>KSCPSVCRCDAGFIYCNDRSLTSIPVGIPEDATTLYLQNNQINNVGIPSDLKNLLKVQRIYLYHNSLDEFPTNLPKYVKELHLQENNIRTITYDSLSKIPYLEELHLDDNSVSAVSIEEGAFRDSNYLRLLFLSRNHLSTIPGGLPRTIEELRLDDNRISTISSPSLHGLTSLKRLVLDGNLLNNHGLGDKVFFNLVNLTELSLVRNSLTAAPVNLPGTSLRKLYLQDNHINRVPPNAFSYLRQLYRLDMSNNNLSNLPQGIFDDLDNITQLILRNNPWYCGCKMKWVRDWLQSLPVKVNVR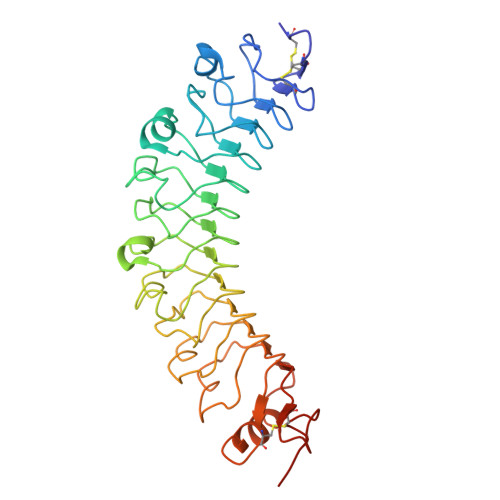GLMCQAPEKVRGMAIKDLSAELFDCKDSG[2x]>[4x]MNGPQTRESLANEIWRACDIMRRDNNCTGIMEYVEHLAWLLFLRFLDAQEEE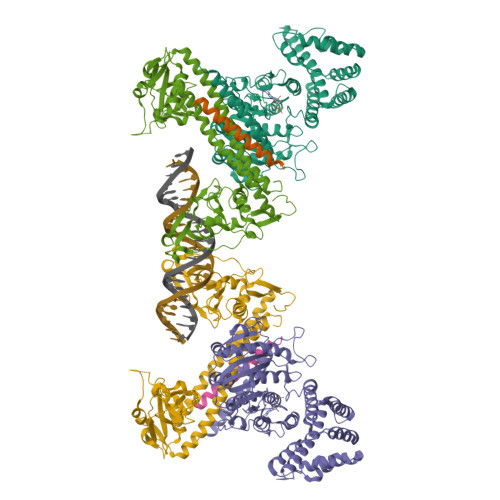WEAQAQIAGRPYTPIIDSEYRWRHWATKDWPADELLAFVHGRLIPYLRSLGGDPLRETIRSLFSERNVIVCASGYNLKDVIQIVNEINFHSQDDIFTVSQVYEELLRRLGNENRLAGEFYTPRPVVRFVVELVDPQIGEAVYDPACGTCGFLVEAYLWMKQKERTIEDHRILQERTFFGQEKKPVPAFLGLVNMMLHGVTVPRVMRRNTLEENIRNVSERFDVVVTNPPFGGTEGRHIQQNFPIQSNATELLFLQHIMKKLKPRDGARCGMVVPEGTLFRGGAFAEVKRDLLEQFNLHTVVSLPPGTFAPYSDVKTALIFFERPGPTKEIWYYELPLPEGLKKFSKGNPIQDEHFEEARKLWRGWDAYRKGLGPVEACLSERSWIVPVEEVKKRGYDLTARNPNRSGGEELPSPVEIVAGLLEKEREILSIMEELSELLENEKGNSSRKNDEEEE;>VTEGPYKLPPGWRWVRLGEVCLPTERRDPTKNPSTYFVYVDISAIDSTVGKIVSPKEILGQHAPSRARKVIRSGDVIFATTRPYLKNIALVPPDLDGQICSTGFCVIRANREFAEPEFLFHLCRSDFITNQLTASKMRGTSYPAVTDNDVYNTLIPLPPLEEQRRIVAKVEALMERVREVRRLRAEAQKDTELLMQTALAEVFPHPGADLPPGWRWVRLGEVCDIIMGQSPPSSTYNFEGNGLPFFQGKADFGDLHPTPRIWCSAPQKVARPGDVLISVRAPVGSTNVANLACCIGRGLAALRPRDSLERFWLLYYLHYLEPELSKMGAGSTFNAITKKDLQNVFIPLPPLEEQRRIVAYLDQIQQQVAALKRAQAETEAELKRLEQAILDKAFRGDL[2x]> MKLQREVYIAGVGETKFGKHTVDFDVLGREAALQAMNGSNIDRP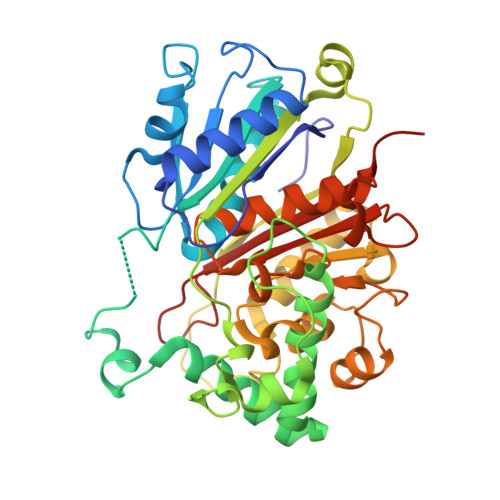DMIQSAYVGNGMNDMTTGQAVFRGLGMCGPNLPIINVQSACSAGAMAVFCAIKDVATGVTDLSIGVGTENHTMHRQSGAAFSAARSDIETMHGAVMTGKYAMRATRYMHETGATIEDLAMITVKNRKHATHNPYAWFKGAITVEEVVNSRMVAYPMTLQQCCGIADGAAAVVVGSKEMMKKLGIAKPVKVAGVVVESGPYHNRPRDITGDDITETTSEKLYEESGIGPKEVNILELHDAFTIAELLYYECMGLCKKGDGLKFLRDGQSTYGGQCVVSPRGGLLSYGHPIGASGAAQIAQNVKQLRGECGGYQVGPTPKVAMSHVTGGGLSGTEHAACTMHMLVKGWGS> LKESPSGYLRSGEGDTGCGELVWVGEPLTLRTAETITGKYGVWMRDPKPTYPYTQETTWRIDTVGTDVRQVFEYDLISQFMQGYPSKVHILPRPLESTGAVVYSGSLYFQGAESRTVIRYELNTETVKAEKEIPGAGYHGQFPYSWGGY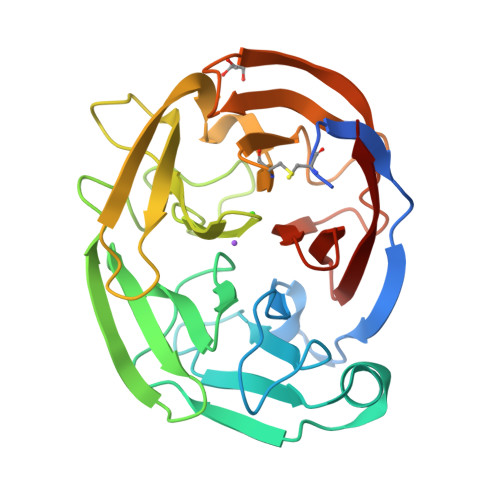TDIDLAVDEAGLWVIYSTDEAKGAIVLSKLNPENLELEQTWETNIRKQSVANAFIICGTLYTVSSYTSVDATVNFAYDTGTGISKTLTIPFKNRYKYSSMIDYNPLEKKLFAWDNLNMVTYDIKLSKM Dichelobacter nodosus is a Gram negative, anaerobic rod that is the principal causative agent of ovine footrot, a debilitating disease of the hoof of ruminants. In strains that cause virulent footrot these proteases are called acidic protease isoenzymes 2 and 5 from virulent strains (AprV2 and AprV5) and basic protease from virulent strains (BprV). All of these proteases are synthesised as inactive precursors with an N-terminal pre-pro-region, a serine protease domain and a C-terminal domain of unknown function. AprV2 adopts a subtilisin-like fold consisting of a curved six-stranded parallel beta sheet sandwiched between two and five alpha helices.

Sequence analysis of the aprV2 and aprB2 genes has shown there is only one amino acid difference (Y92R) between the two mature proteases. To investigate how the single amino acid difference (Y92R) between the active forms of AprV2 and AprB2 alters the substrate specificity of AprB2 we determined the crystal structures of AprV2 and AprB2 to 2.0 Å and 1.7 Å, respectively. The two structures were very similar (RMSD of 0.28 Å for 339 Cα) and therefore we will describe the structure with reference to AprV2. Surprisingly, the single amino acid difference between AprV2 and AprB2 (Y92R) is located at the tip of this extended loop, ∼27 Å from the active site serine (S277). Purified AprB2, which differs in sequence from AprV2 only at residue 92, is less efficient at degrading elastin. Under these conditions, the ability of AprB2 to degrade the substrate was significantly less than AprV2 (p<0.05). Both proteases displayed similar activity against the soluble chromogenic elastase substrate, N-Methoxysuccinyl-Ala-Ala-Pro-Val p-nitroanilide (AAPVn), with kinetic parameters that were of the same order of magnitude. Instead, the reduced elastinolytic activity of AprB2 is likely to arise from impaired enzyme-substrate interactions at a site distal to the active site. To our surprise, complementation of the aprV2 mutant with aprB2 also restored a virulent phenotype, indicating that AprV2-mediated elastase activity was not required for virulence. Importantly, the hoof digestion pattern produced by AprB2 was similar to that produced by AprV2, which is consistent with results of the virulence trials.

> APNDQHYREQWHYFDRYGVKADKVWDMGFTGQNVVVAVVDTGILHHRDLNANVLPGYDFISNSQISLDGDGRDADPFDEGDWFDNWACGGRPDPRKERSDSSWHGSHVAGTIAAVTNNRIGVAGVAYGAKVVPVRALGRCGGYDSDISDGLYWAAGGRIAGIPENRNPAKVINMSLGSDGQCSYNAQTMIDRATRLGALVVVAAGNENQNASNTWPTSCNNVLSVGATTSRGIRASFSNYGVDVDLAAPGQDILSTVDSGTRRPVSDAYSFMAGTSMATPHVSGVAALVISAANSVNKNLTPAELKDVLVSTTSPFNGRLDRALGSGIVDAEAAVNSVLG> MRVLVTGG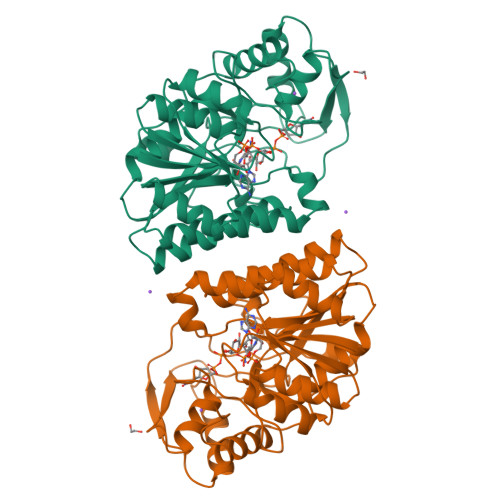SGYIGSHTCVQLLQNGHDVIILDNLCNSKRSVLPVIERLGGKHPTFVEGDIRNEALMTEILHDHAIDTVIHFAGLKAVGESVQKPLEYYDNNVNGTLRLISAMRAANVKNFIFSSAATVYGDNPKIPYVESFPTGTPQSPYGKSKLMVEQILTDLQKAQPDWSIALLRYFNPVGAHPSGDMGEDPQGIPNNLMPYIAQVAVGRRDSLAIFGNDYPTEDGTGVRDYIHVMDLADGHVVAMEKLANKPGVHIYNLGAGVGNSVLDVVNAFSKACGKPVNYHFAPRREGDLPAYWADASKADRELNWRVTRTLDEMAQDTWHWQSRHPQGYPD> ACPPC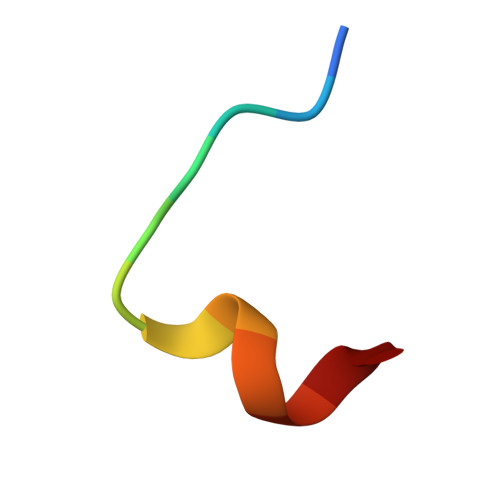LWQVLCG>[6x]VETISFSFSEFEPGNDNLTLQGASLITQSGVLQLTKINQNGMPAWDSTGRTLYAKPVHIWDMTTGTVASFETRFSFSIEQPYTR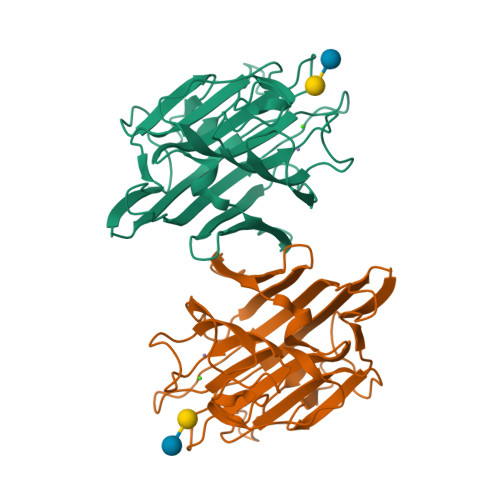PLPADGLVFFMGPTKSKPAQGYGYLGIFNNSKQDNSYQTLGVEFDTFSNQWDPPQVPHIGIDVNSIRSIKTQPFQLDNGQVANVVIKYDASSKLLHAVLVYPSSGAIYTIAEIVDVKQVLPEWVDVGLSGATGAQRDAAETHDVYSWSFQASLPE> MRGSHHHHHHGLVPRGSMIRTMLQGKLHR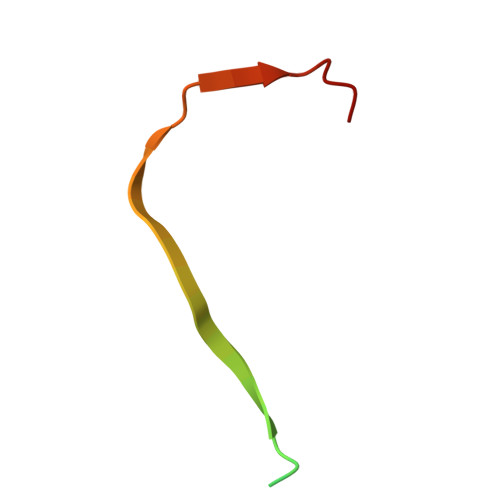VKVTHADLHYEG> CTKSIPPQ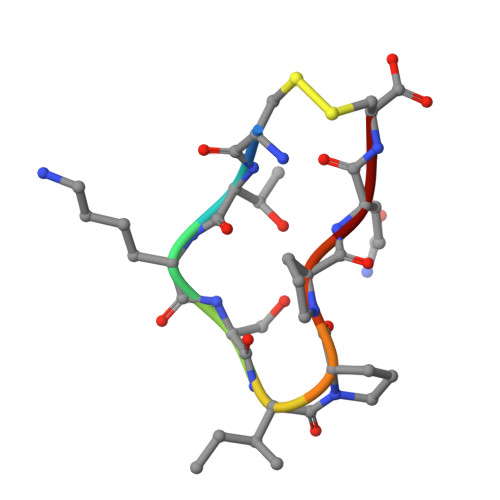C>[8x]GPGSSGPADCCRMKECCTDRVNECLQRYSG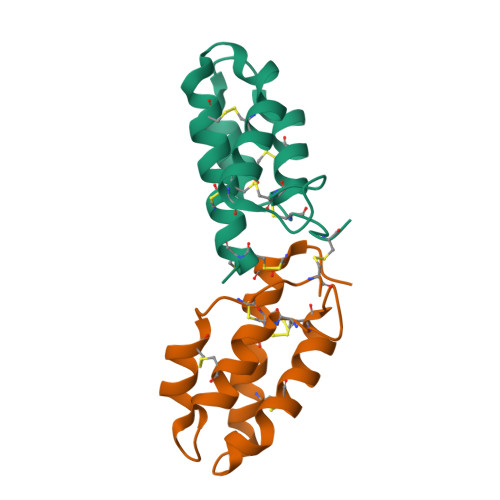REDKFVSFCYQEATVTCGSFNEIVGCCYGYQMCMIRVVKPNSLSGAHEACKTVSCGNPCA> MVVTRIAPSPTGDPHVGTAYIALFNYAWARRNGGRFIVRIEDTDRARYVPGAEERILAALKWLG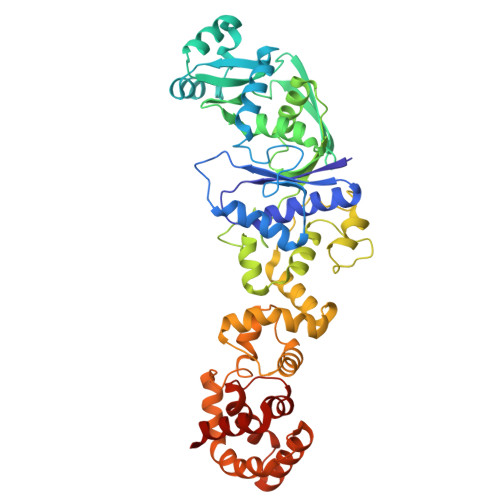LSYDEGPDVAAPTGPYRQSERLPLYQKYAEELLKRGWAYRAFETPEELEQIRKEKGGYDGRARNIPPEEAEERARRGEPHVIRLKVPRPGTTEVKDELRGVVVYDNQEIPDVVLLKSDGYPTYHLANVVDDHLMGVTDVIRAEEWLVSTPIHVLLYRAFGWEAPRFYHMPLLRNPDKTKISKRKSHTSLDWYKAEGFLPEALRNYLCLMGFSMPDGREIFTLEEFIQAFTWERVSLGGPVFDLEKLRWMNGKYIREVLSLEEVAERVKPFLREAGLSWESEAYLRRAVELMRPRFDTLKEFPEKARYLFTEDYPVSEKAQRKLEEGLPLLKELYPRLRAQEEWTEAALEALLRGFAAEKGVKLGQVAQPLRAALTGSLETPGLFEILALLGKERALRRLERALA>PHMSGLKKFFPYSTNVLKGAAADIALPSLAGKTVFFYFSASWCPPCRAFTPQLIDFYKAHAEKKNFEVMLISWDESAEDFKDYYAKMPWLALPFEDRKGMEFLTTGFDVKSIPTLV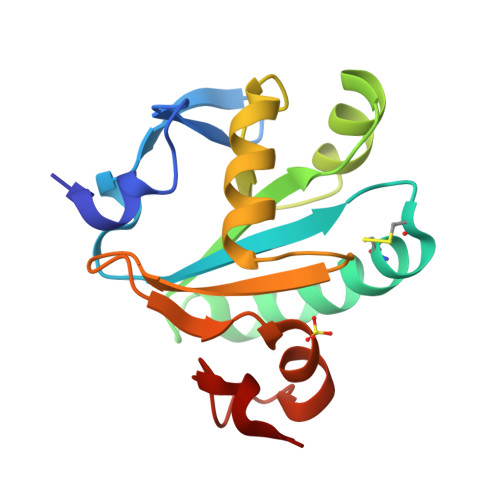GVEADSGNIITTQARTMVVKDPEAKDFPWPNVEAKK[2x]>VTPPPEKFNFAEHLLQTNRVRPDKTAFVDDISSLSFAQLEAQTRQLAAALRAIGVKREERVLLLMLDGTDWPVAFLGAIYAGIVPVAVNTLLTADDYAYMLEHSRAQAVLVSGALHPVLKAALTKSDHEVQRVIVSRPAAPLEPGEVDFAEFVGAHAPLEKPAATQADDPAFWLYSSGSTGRPKGVVHTHANPYWTSELYGRNTLHLREDDVCFSAAKLFFAYGLGNALTFPMTVGATTLLMGERPTPDAVFKRWLGGVGGVKPTVFYGAPTGYAGMLAAPNLPSRDQVALRLASSAGEALPAEIGQRFQRHFGLDIVDGIGSTEMLAAFLSNLPDRVRYGTTGWPVPGYQIELRGDGGGPVADGEPGDLYIHGPSSATMYWGNRAKSRDTFQGGWTKSGDKYVRNDDGSYTYAGRTDDMLKVSGIYVSPFEIEATLVQHPGVLEAAVVGVADEHGLTKPKAYVVPRPGQTLSETELKTFIKDRLAPYKYPRSTVFVAELPKTATGKIQRFKLREGVL[2x]

BadA catalyzes the conversion of benzoate to benzoyl-CoA in the metabolism of aromatic carboxylic acids. Its catalytic mechanism is shown as follows: benzoate firstly docks to the active site, where it orientates to allow the carboxylic group access to adenosine triphosphate (ATP) for the formation of an adenosine monophosphate (AMP) intermediate; coenzyme A (CoA) subsequently comes in to substitute the AMP-activated intermediate resulting in the formation of benzoyl-CoA. The solved structures show that the benzoate binding cavity is rather small and narrow, constituted by several bulky amino acid residues including Y228, G327, S328, T329, H333, and I334. With the purpose to allow acceptance of various bulkier substrates into the active site, a double mutant H333A and I334A was created.

The capability and capacity of the engineered benzoate-CoA ligase are manifested by crystal structures in complex with a 2-chloro-1,3-thiazole-5-carboxyl-AMP or 2-methlthiazole-5-carboxyl-AMP intermediate. As revealed from the determined complexes, there are considerable hydrophobic contacts between substrates and the polypeptide backbone of the BadA active site. In AMP binding site, Lys427 plays an important role in coordination with the carboxylate group of the ligand by its positive charge and in stabilization with the AMP group during the thioesterification. Several residues in the AMP binding site, including Arg421, Thr329, Ser328, Gly303, Asp406, Asp324, Asp325, with polar contacts with the AMP-linked intermediate together stabilize the intermediate for subsequent thioesterification to proceed. The crystal structures of the BadA mutant (H333A/I334A) in complex with two different intermediates validated the objectivity and rationality of this modification. Three protein crystal structures in an apo form and in complex with a 2-methylthiazole-5-carboxyl-AMP or 2-choloro-1,3-thiazole-5-carboxyl-AMP intermediate validated the engineering rationality and synthetic practicality of the modified enzyme. To further explore/expand the substrate promiscuity of P. sylvestris STS, five different thaizole CoA derivatives 4-methylthiazole-5-carboxyl-CoA, 2-methylthiazole-5-carboxyl-CoA, 2-chloro-1,3-thiazole-5-carboxyl-CoA, 2-bromothiazole-4-methyl-5-carboxyl-CoA (2Br4M5C-CoA), 2-bromothiazole-5-methyl-4-carboxyl-CoA (2Br5M4C-CoA) were enzymatically synthesized using the engineered BadA, which were then subjected to biochemical examination.> MEIPVIEPLFTKVTEDIPGAEGPVFD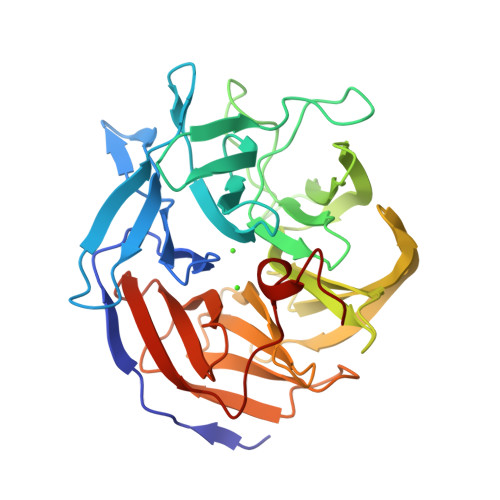KNGDFYIVAPEVEVNGKPAGEILRIDLKTGKKTVICKPEVNGYGGIPAGCQCDRDANQLFVADMRLGLLVVQTDGTFEEIAKKDSEGRRMQGCDDCAFDYEGNLWITAPAGEVAPADYTRSMQEKFGSIYCFTTDGQMIQVDTAFQFPDGIAVRHMNDGRPYQLIVAETPTKKLWSYDIKGPAKIENKKVWGHIPGTHEGGANGMDFDEDNNLLVANWGSSHIEVFGPDGGQPKMRIRCPFEKPSNLHFKPQTKTIFVTEHENNAVWKFEWQRNGKKQYCETLKFGIF>HHHHHHENLYFQGSGSSPRSGVLLRGCPTHCHCEPDGRMLLRVDCSDLGLSELPSNLSVFTSYLDLSMNNISQLLPNPLPSLRFLEELRLAGNALTYIPKGAFTGLYSLKVLMLQNNQLRHVPTEALQNLRSLQSLRLDANHISYVPPSCFSGLHSLRHLWLDDNALTEIPVQAFRSLSALQAMTLALNKIHHIPDYAFGNLSSLVVLHLHNNRIHSLGKKCFDGLHSLETLDLNYNNLDEFPTAIRTLSNLKELGFHSNNIRSIPEKAFVGNPSLITIHFYDNPIQFVGRSAFQHLPELRTLTLNGASQITEFPDLTGTANLESLTLTGAQISSLPQTVCNQLPNLQVLDLSYNLLEDLPSFSVCQKLQKIDLRHNEIYEIKVDTFQQLLSLRSLNLAWNKIAIIHPNAFSTLPSLIKLDLSSNLLSSFPITGLHGLTHLKLTGNHALQSLISSENFPELKVIEMPYAYQCCAFGVCENAYKISNQWNKGDNSSMDDLHKKDAGMFQAQDERDLEDFLLDFEE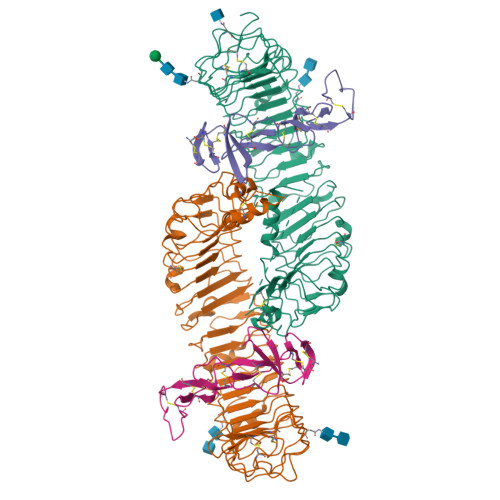DLKALHSVQCSPAAA[2x];>GSRISAEGSQACAKGCELCSEVNGCLKCSPKLFILLERNDIRQVGVCLPSCPPGYFDARNPDMNKCIKCKIEHCEACFSHNFCTKCKEGLYLHKGRCYPACPEGSSAANGTMECSSPAAAHHHHHH[2x]>MSDATKRPLRADAQRNRDKILAAAVRVFSEEGLDAHLERIAREAGVGSGTLYRNFPTREALIEAAYRNEVARLCDSVPGLLAELPPAEALRAWTRRFIDYATAKLGMADALRAVVASGGDPYGDSRQLIQSALTALMDAAAAAGEIRSDIRSTDMFAALAGIALTSSRPDQR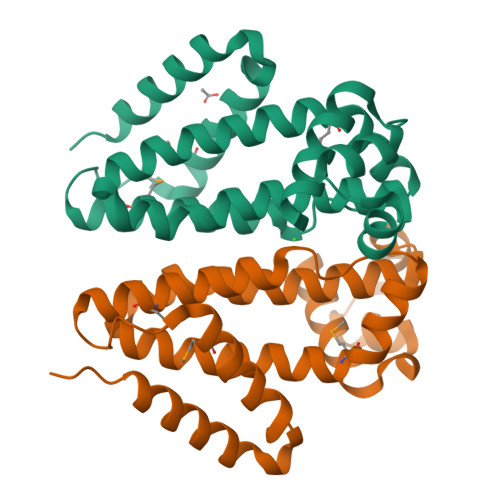AQAERLLDLVLDGLRPTAPRPA[2x]>ASAKLPGDFGPPRGEPIHAVLTSPPLVPPPVNRTYPAKVIVELEVVEKEMQISEGVSYTFWTFGGTVPGSFIRVRQGDTVEFHLKNHPSSKMPHNIDLHGVTGPGGGAASSFTAPGHESQFTFKALNEGIYVYHCATAPVGMHIANGMYGLILVEPPEGLPKVDHEYYVMQGDFYTAGKYREKGLQPFDMEKAIDERPSYVLFNGAEGALTGDKALHAKVGETVRIFVGNGGPNLVSSFHVIGAIFDQVRYEGGTNVQKNVQTTLIPAGGAAVVKFTARVPGSYVLVDHSIFRAFNKGAMAILKIDGAENKLVYSGKELDSVELGDRAAPNMSAVTKATQASVSGTLTVQDQVQAGRALFAGTCSVCHQGNGAGLPGVFPPLAKSDFLAADPKRAMNIVLHGLNGKIKVNGQEYDSVMPPMTQLNDDEVANILTYVLNSWDNPGGRVSAEDVKKVRAQPAPAKAVAEH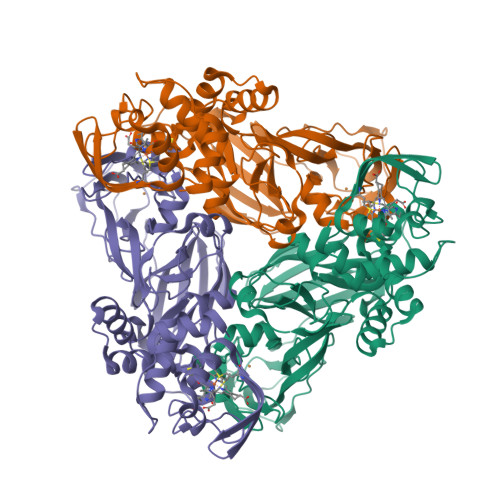[2x]> MGMEEIEHRTVEVNGIKMHV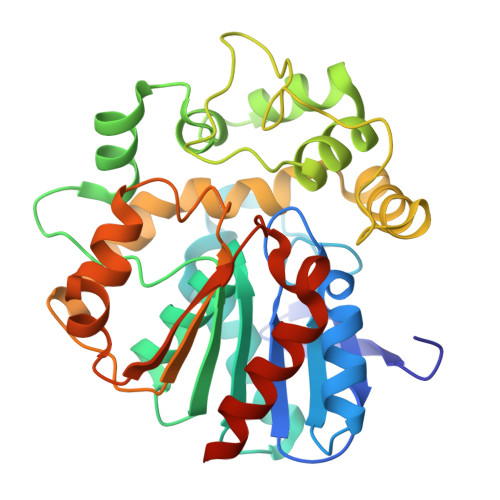AEKGEGPVVLFLHGFPELWYSWRHQILALSSRGYRAVAPDLRGYGDTEAPVSISSYTGFHIVGDLIALIDLLGVDQVFLVAHDWGAIIGWYLCTFHPDRVKAYVCLSVPLLHRDPNIRTVDAMRAMYGDDYYICRFQKPGEMEAQMAEVGTEYVLKNILTTRKPGPPIFPKGEYGTGFNPDMPNSLPSWLTQDDLAYYVSKYEKTGFTGPLNYYRNMNLNWELTAPWSGGKIQVPVKFITGELDQVYTSLNMKEYIHGGGFKQDVPNLEEVIVQKNVAHFNNQEAAEEINNHIYDFIKKFLQHHHHHH> IMTDAFQTAESREVTGAQGFAPTEGESIVLSHNIQHQVALPPDLDYEYIPLSEHKPPAEPARTYSFKLDPFQALSVASIEREESVLVSAHTSAGKTVVAEYAIAQCLKKNQRVIYTSPIKALSNQKYRDFQAEFGDVGLMTGDVTINPTASCLVMTTEILRSMLYRGSEIMREVAWVVFDEIHYMRDKIRGVVWEETIILLPDKVRYVFLSATIPNAFQFAEWIAKIHRQACHVVYTDFRPTPLQNYFFPAGGKGILLIVDEKGNFKENNFNQAMAMIEEKKGTDSNDWSAKQKGKGKNKKTNKGGEAADEKADIAKIIKMILKKNFQPVIVFNFSKRECEQMALASSSMKFNAPDEENMVNKVFENALASLSEDDKNLPQISNILPLLRKGIGVHHSGLLPILKETIEILFQEGLIKVLFATETFSIGLNMPARTVVFTQVTKWDGQQRRPLTSSEYIQMAGRAGRRGLDDRGIVIMMVDDKLEPETARAIVVGNQDKLNSAFHLGYNMVLNLLRIEAISPEYMLERCFFQFQNAASVPQLERELISLQQERDAIIIPDESIVKDYYGVRQQLEEYNKDMVFVIQHPQNCLGFFQEGRLIHIKSPSGVDYGWGVLIKHIQRQTPKNGQPPYPEQESYVLDVLLKVSGDFNPKTRGEGPMPEGIMPAGKDSKNARWEVVPCLLNCLRALGQLRVFLPKRLESADEKDGVGKAVDEISRRFPDGIPILDPMENMGINDDSFKKLLRKIEVLESRLVANPLHNSPLLVELWNQYSLKMQLGEQIKEKKKAIARAHSVAQLDELKSRKRVLRRLGFINDAEVVQMKARVACEISSTEGHELLLAELLFNRFFNELSPEICACILSCFIFDEKIETQALKEELAKPFREIQAQARIIAKVSAESKLDVNEDEYVQSLKWQLMETVLAWAQGRPFSEICKMT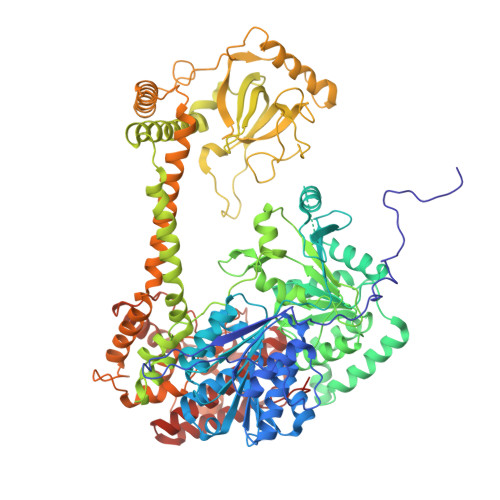NVYEGSLIRLFRRLEELLRQMAEAARVMGSEELKDKFELSLSKIRRDIVSFNSLYL>MAGKEIQTPDQAEAFVAKVFDVLDSYDYTRFGEVLSTDLKYEGGLQKTSGLDNFINDIKASTQRMPGLQTSHSRYRTELTAEGTIYSEGHSNASLESNPGKVVTVPMIGVF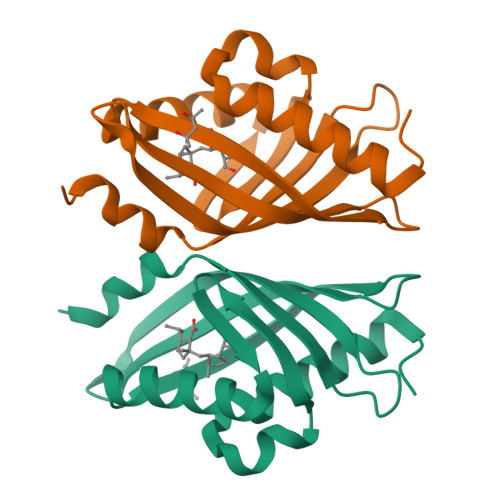KLDSEDGKIKEMRIYKDRLPFLALHQALPGMKANN[2x]> MAGFWVGTAPLVAAGRRGRWPPQQLMLSAALRTLKHVLYYSRQCLMVSRNLGSVGYDPNEKTFDKILVANRGEIACRVIRTCKKMGIKTVAIHSDVDASSVHVKMADEAVCVGPAPTSKSYLNMDAIMEAIKKTRAQAVHPGYGFLSENKEFARCLAAEDVVFIGPDTHAIQAMGDKIESKLLAKKAEVNTIPGFDGVVKDAEEAVRIAREIGYPVMIKASAGGGGKGMRIAWDDEETRDGFRLSSQEAASSFGDDRLLIEKFIDNPRHIEIQVLGDKHGNALWLNERECSIQRRNQKVVEEAPSIFLDAETRRAMGEQAVALARAVKYSSAGTVEFLVDSKKNFYFLEMNTRLQVEHPVTECITGLDLVQEMIRVAKGYPLRHKQADIRINGWAVECRVYAEDPYKSFGLPSIGRLSQYQEPLHLPGVRVDSGIQPGSDISIYYDPMISKLITYGSDRTEALKRMADALDNYVIRGVTHNIALLREVIINSRFVKGDISTKFLSDVYPDGFKGHMLTKSEKNQLLAIASSLFVAFQLRAQHFQENS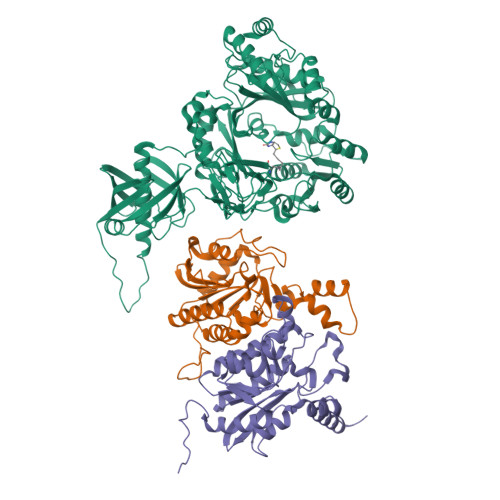RMPVIKPDIANWELSVKLHDKVHTVVASNNGSVFSVEVDGSKLNVTSTWNLASPLLSVSVDGTQRTVQCLSREAGGNMSIQFLGTVYKVNILTRLAAELNKFMLEKVTEDTSSVLRSPMPGVVVAVSVKPGDAVAEGQEICVIEAMKMQNSMTAGKTGTVKSVHCQAGDTVGEGDLLVELE;> DPSDRLVPELDTIVPLESTKAYNMVDIIHSVVDEREFFEIMPNYAKNIIVGFARMNGRTVGIVGNQPKVASGCLDINSSVKGARFVRFCDAFNIPLITFVDVPGFLPGTAQEYGGIIRHGAKLLYAFAEATVPKVTVITRKAYGGAYDVMSSKHLCGDTNYAWPTAEIAVMGAKGAVEIIFKGHENVEAAQAEYIEKFANPFPAAVRGFVDDIIQPSSTRARICCDLDVLASKKVQRPWRKHANIPL;> MAAALRVAAVGARLSVLASGLRAAVRSLCSQATSVNERIENKRRTALLGGGQRRIDAQHKRGKLTARERISLLLDPGSFVESDMFVEHRCADFGMAADKNKFPGDSVVTGRGRINGRLVYVFSQDFTVFGGSLSGAHAQKICKIMDQAITVGAPVIGLNDSGGARIQEGVESLAGYADIFLRNVTASGVIPQISLIMGPCAGGAVYSPALTDFTFMVKDTSYLFITGPDVVKSVTNEDVTQEELGGAKTHTTMSGVAHRAFENDVDALCNLRDFFNYLPLSSQDPAPVRECH> MRRYEVNIVLNPNLDQSQLALEKEIIQRALENYGARVEKVAILGLMVLAYPIAKDPQGYFLWYQVEMPE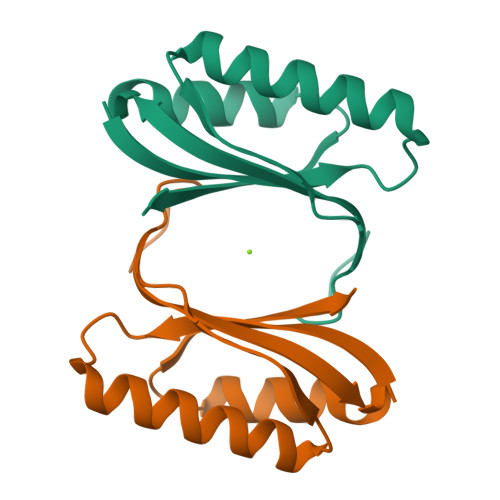DRVNDLARELRIRDNVRRVMVVKSQEPFLANA> ADLADRFAELERRYDARLGVYVPATGTTAAIEYRADERFAFCSTFKAPLVAAVLHQNPLTHLDKLITYTSDDIRSISPVAQQHVQTGMTIG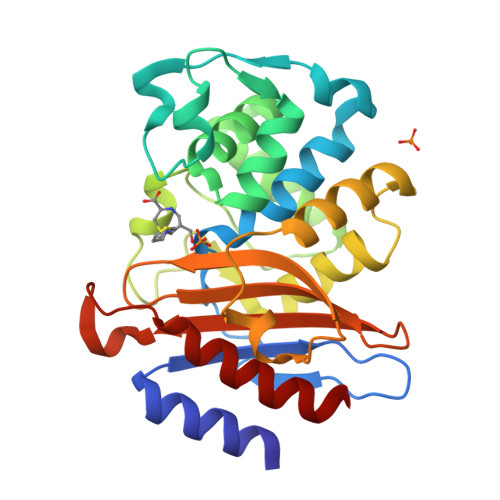QLCDAAIRYSDGTAANLLLADLGGPGGGTAAFTGYLRSLGDTVSRLDAEEPELNRDPPGDERDTTTPHAIALVLQQLVLGNALPPDKRALLTDWMARNTTGAKRIRAGFPADWKVIDKTGTGDYGRANDIAVVWSPTGVPYVVAVMSDRAGGGYDAEPREALLAEAATCVAGVLA2-[(5~{E})-5-[[3-[4-(2-fluoranylphenoxy)phenyl]-1-phenyl-pyrazol-4-yl]methylidene]-4-oxidanylidene-2-sulfanylidene-1,3-thiazolidin-3-yl]ethanesulfonic 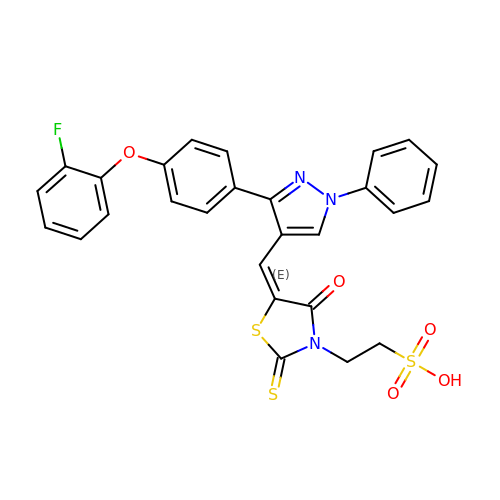acid | C27 H20 F N3 O5 S3 | JNBMBOFCJMRUHR-LFVJCYFKSA-N> MGMLELVGEYWEQLKITVVPVVAAAEDDDNEQHEEKAAEGEEKEEENGDEDEDEDEDEDDDDD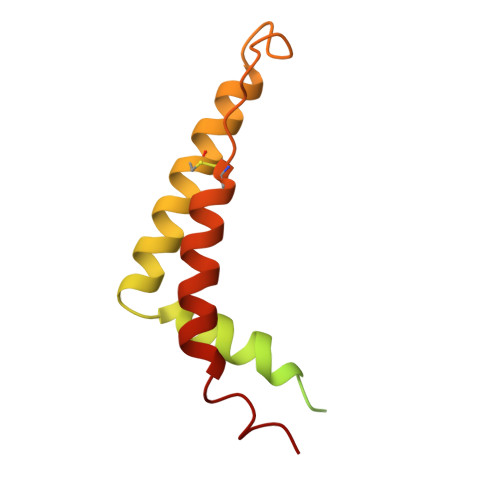DDEDEEEEEEVTDQLEDLREHFKNTEEGKALVHHYEECAERVKIQQQQPGYADLEHKEDCVEEFFHLQHYLDTATAPRLFDKLK>MASMTGGQQMGRGSMSRDPLPFFPPLYLGGPEITTENCEREPIHIPGSIQPHGALLTADGHSGEVLQMSLNAATFLGQEPTVLRGQTLAALLPEQWPALQAALPPGCPDALQYRATLDWPAAGHLSLTVHRVGELLILEFEPTEAWDSTGPHALRNAMFALESAPNLRALAEVATQTVRELTGFDRVMLYKFAPDATGEVIAEARREGLHAFLGHRFPASDIPAQARALYTRHLLRLTADTRAAAVPLDPVLNPQTNAPTPLGGAVLRATSPMHMQYLRNMGVGSSLSVSVVVGGQLWGLIACHHQTPYVLPPDLRTTLEYLGRLLSLQVQVKEAADVAAFRQSLREHHARVALAAAHSLSPHDTLSDPALDLLGLMRAGGLILRFEGRWQTLGEVPPAPAVDALLAWLETQPGALVQTDALGQLWPAGADLAPSAAGLLAISVGEGWSECLVWLRPELRLEVAWGGATPDQAKDDLGPRHSFDTYLEEKRGYAEPWHPGEIEEAQDLRDTLTGALGERLSVIRDLNRALTQSNAEWRQYGFVISHHMQEPVRLISQFAELLTRQPRAQDGSPDSPQTERITGFLLRETSRLRSLTQDLHTYTALLSAPPPVRRPTPLGRVVDDVLQDLEPRIADTGASIEVAPELPVIAADAGLLRDLLLHLIGNALTFGGPEPRIAVRTERQGAGWSIAVSDQGAGIAPEYQERIFLLFQRLGSLDEALGNGLGLPLCRKIAELHGGTLTVESAPGEGSTFRCWLPDAGPLPGAADAASSAGGSAGSAGMPERASVPLRLLLVEDNAADIFLMEMALEYSSVHTELLVARDGLEALELLEQAKTGGPFPDLILLDLNMPRVDGFELLQALRADPHLAHLPAIVLTTSNDPSDVKRAYALQANSYLTKPSTLEDFLQLIERLTAYWFGTAAIPQTYQPQLEHHHHHH[2x]

Phytochromes are a protein superfamily in bacteria, plants, and fungi, and function by photoswitching between states that absorb red light (Pr) and far-red light (Pfr). Conserved over the entire superfamily and exemplified by the phytochrome from D. radiodurans, phytochromes share a photosensory core module, consisting of PAS, GAF, and PHY domains and a bilin chromophore, which is connected to a variable effector module via helical linkers. Many bacteriophytochromes are histidine kinases or phosphatases in two-component systems (TCSs). For the single-particle cryo-EM experiment, we used a fusion of DrBphP with its response regulator protein (abbreviated DrBphP-DrRR) via a 12 amino acid tether.

Homogeneous refinement of class 1 followed by local refinement implemented in cryoSPARC v3.1.0 gave a resolution of 3.6 Å, and local refinement with a mask over the PAS-GAF-PHY-neck region resulted from a resolution of 3.4 Å. The modeled structure shows the signatures expected for the Pr state, including the PHY tongue in a β-sheet conformation and the biliverdin in 15Z conformation. The structure of the PAS-GAF-PHY domains is almost identical to the crystal structure of the corresponding truncation of DrBphP. The cryo-EM structures presented here are free of these biases. They firmly confirm a head-to-head arrangement of the dimer for bacterial phytochromes and indicate that the bent conformation of the photosensory core module previously detected in Pr crystals is the one that is present in the solution.> GGSGGSGGSGGSGGSPTNYEYDEASETWPSFILTGLLMVVGPMTLLQIYQIFFGANAEDGNSGKSKEFNEEVFKNLNEEYTSDEIKQFRRKFDKNSNKKSKIWSRRNIIIIVGWILVAILLQRINSNDAIKDAATKLFDPYEILGISTSASDRDIKSAYRKLSVKFHPDKLAKGLTPDEKSVMEETYVQITKAYESLTDELVRQNYLKYGHPDGPQSTSHGIALPRFLVDGSASPLLVVCYVALLGLILPYFVSRWWARTQSYTKKGIHNVTASNFVSNLVNYKPSEIVTTDLILHWLSFAHEFKQFFPDLQPTDFEKLLQDHINRRDSGKLNNAKFRIVAKCHSLLHGLLDIACGFRNLDIALGAINTFKCIVQAVPLTPNCQILQLPNVDKEHFITKTGDIHTLGKLFTLEDAKIGEVLGIKDQAKLNETLRVASHIPNLKIIKADFLVPGRPYISLKVLVRSAKQPLIPTSLIPEENLTEPQDSESQRDPFAMMSKQPLVPYSFAPFFPTKRRGSWCCLVSSQKDGKILQTPIIIEKLSYKNLNDDKDFFDKRIKMDLTKHEKFDINDW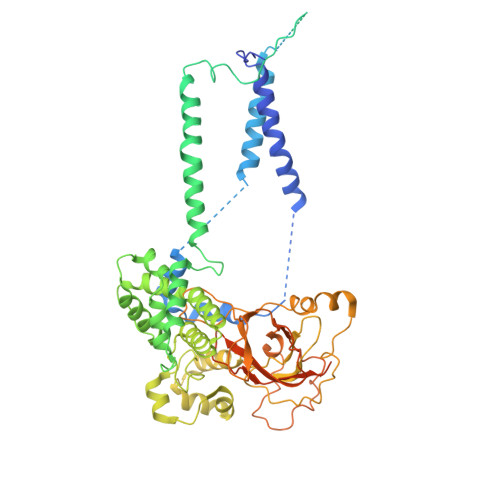EIGTIKIPLGQPAPETVGDFFFRVIVKSTDYFTTDLDITMNMKVRDSPAVEQVEVYSEEDDEYSTDDDETESDDESDASDYTDIDTDTEAEDDESPEGENLYFQ> MSPFPLTSMDKAFITVLEMTPVLGTEIINYRDGMGRVLAQDVYAKDNLPPFPASVKDGYAVRAADGPGDRFIIGESQAGEQPTQTVMPGQVMRVTTGAPIPCGADAVVQVEDTELIRESDDGTEELEVRILVQARPGQDIRPIGHDIKRGECVLAKGTHMGPSEIGLLATVGVTEVEVNKFPVVAVMSTGNELLNPEDDLLPGKIRDSNRSTLLATIQEHGYPTINLGIVGDNPDDLLNALNEGISRADVIITSGGVSMGEKDYLKQVLDIDLHAQIHFGRVFMKPGLPTTFATLDIDGVRKIIFALPGNPVSAVVTCNLFVVPALRKMQGILDPRPTIIKARLSCDVKLDP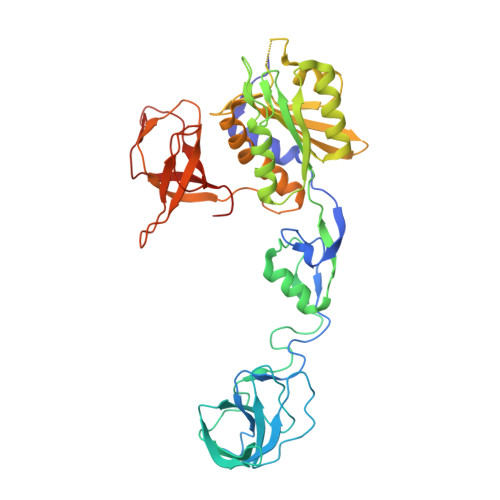RPEYHRCILTWHHQEPLPWAQSTGNQMSSRLMSMRSANGLLMLPPKTEQYVELHKGEVVDVMVIGRL>CCGTTAACGG[2x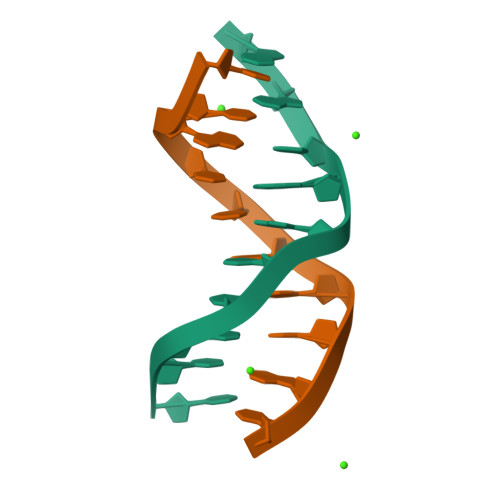]In previous work, we have introduced pAF into lactococcal multidrug resistance regulator (LmrR), a small homodimeric protein harbouring a pore that exhibits promiscuous substrate binding capabilities, either by direct incorporation using the dedicated orthogonal translation system (OTS),19 or, preferably, by introduction of p-azidophenylalanine (pAzF), followed by a post-translational Staudinger reduction. Incorporation of aY into protein scaffold LmrR gave rise to an artificial Friedel–Crafts (FC) alkylase exhibiting complementary enantioselectivity to a previous FC-alkylase design using p-aminophenylalanine as catalytic residue in the same protein. X-ray crystal structures of the parent and evolved designer enzymes suggest that the introduced mutations cause a narrowing of the active site and a reorientation of the catalytic –NH2 group. Position V15 resides inside the pore of LmrR, and is the same position of ncAA incorporation as used in earlier works featuring pAF as catalytic residue.

We used this improved OTS to incorporate aY via amber SCS at position V15 in the LmrR protein. Remarkably, while V15aY exhibits the characteristic LmrR structure, forming an open pore at its dimeric interface of similar shape and dimensions as observed in other LmrR structures, the V15aY_RNYW_KK structure appears to be more closed and exhibits a narrowed cavity. Furthermore, a significant difference in the rotameric state of the aY side chain is observed (S11†). In the parent structure, the –NH2 group of aY is oriented towards the side of the pore, away from the central W96 and W96′ residues. Strikingly, the opposite enantiomer of product 3a was obtained when compared to LmrR_V15pAF (further referred to as V15pAF), albeit with low yield (entries 2 and 3). The results showed that directed evolution led to a 3.4-fold increase in apparent catalytic efficiency, with (kcat/KM-2a)app values of 3.3 M−1 s−1 and 11.2 M−1 s−1 for V15aY and V15aY_RNYW, respectively.

> GAEIPKEMLRAQTNYILLNVLKQGDNYVYGIIKQVKEASNGEMELNEATLYTIFDRLEQDGIISSYWGDESQGGRRKYYRLTEIGHENMRLAFESWSRVDKIIENLEANKKSEAIKSRGGSGGWSHPQFEK>[4x]NDKLVELSKSDDNWVMPGKNYDSNNFSDLKQINKGNVKQLRPAWTF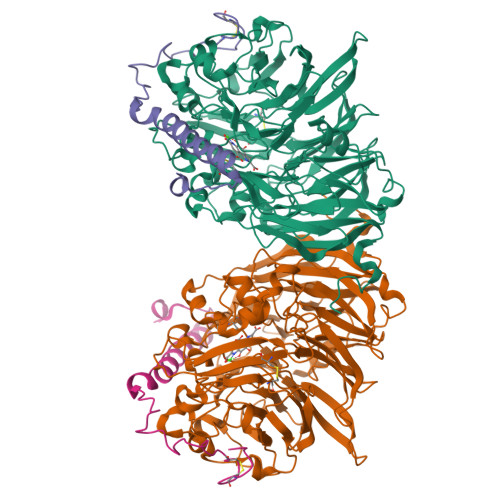STGLLNGHEGAPLVVDGKMYIHTSFPNNTFALGLDDPGTILWQDKPKQNPAARAVACCDLVNRGLAYWPGDGKTPALILKTQLDGNVAALNAETGETVWKVENSDIKVGSTLTIAPYVVKDKVIIGSSGAELGVRGYLTAYDVKTGEQVWRAYATGPDKDLLLASDFNIKNPHYGQKGLGTGTWEGDAWKIGGGTNWGWYAYDPGTNLIYFGTGNPAPWNETMRPGDNKWTMTIFGRDADTGEAKFGYQKTPHDEWEYAGVNVMMLSEQKDKDGKARKLLTHPDRNGIVYTLDRTDGALVSANKLDDTVNVFKSVDLKTGQPVRDPEYGTRMDHLAKDICPSAMGYHNQGHDSYDPKRELFFMGINHICMDWEPFMLPYRAGQFFVGATLNMYPGPKGDRQNYEGLGQIKAYNAITGDYKWEKMERFAVWGGTMATAGDLVFYGTLDGYLKARDSDTGDLLWKFKIPSGAIGYPMTYTHKGTQYVAIYYGVGGWPGVGLVFDLADPTAGLGAVGAFKKLANYTQMGGGVVVFSLDGKGPYDDPNVGEWKSAAK;>YDGTKCKAAGNCWEPKPGFPEKIAGSKYDPKHDPKELNKQADSIKQMEERNKKRVENFKKTGKFEYDVAKISAN[4x]> MENTENSVDSKSIKNLEPKIIHGSESMDSGISLDNSYKMDYPEMGLCIIINNKNFHKSTGMTSRSGTDVDAANLRETFRNLKYEVRNKNDLTREEIVELMRDVSKEDHSKRSSFVCVLLSHGEAGIIFGTNGPVDLKKITNFFRGDRC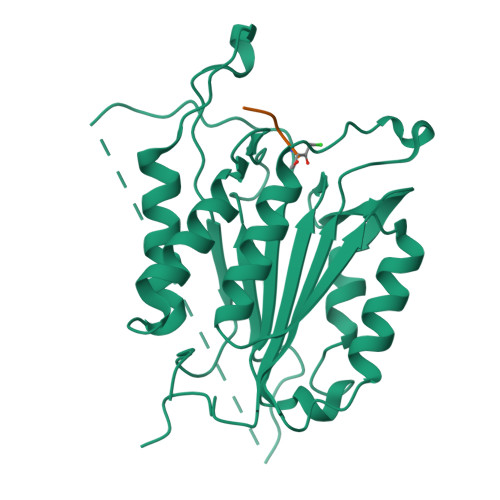RSLTGKPKLFIIQACRGTELDCGIETDSGVDDDMACHKIPVEADFLYAYSTAPGYYSWRNSKDGSWFIQSLCAMLKQYADKLEFMHILTRVNRKVATEFESFSFDATFHAKKQIPCIVSMLTKELYFYH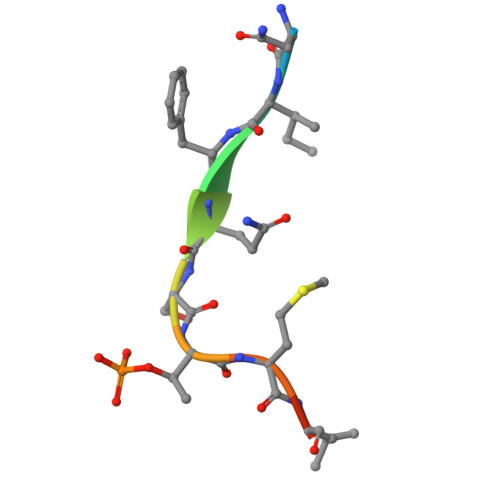> KNIFQSTMLTE>[4x]TEEKTCDLVGEKGKESEKELALLKRLTPLFQKSFESTVGQSPDMYSYV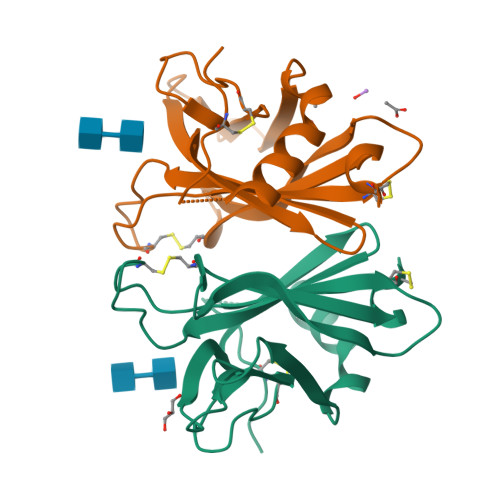FRVCREAGQHSSGAGLVQIQKSNGKETVVGRFNETQIFQGSNWIMLIYKGGDEYDNHCGREQRRAVVMISCNRHTLADNFNPVSEERGKVQDCFYLFEMDSSLACS> RSMAEEVSTLMKATVLMRQPGRVQEIVGALRKGGGDRLQVISDFDMTLSRFAYNG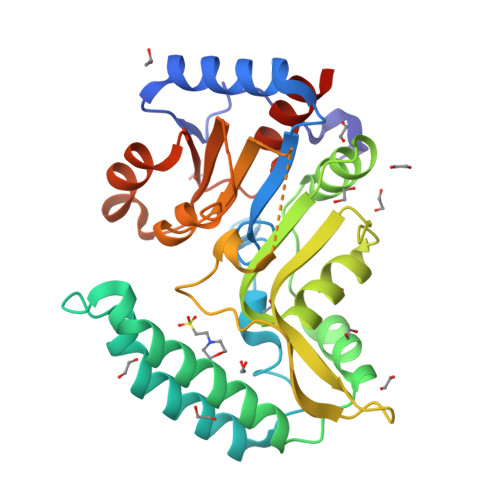KRCPSSYNILDNSKIISEECRKELTALLHHYYPIEIDPHRTVKEKLPHMVEWWTKAHNLLCQQKIQKFQIAQVVRESNAMLREGYKTFFNTLYHNNIPLFIFSAGIGDILEEIIRQMKVFHPNIHIVSNYMDFNEDGFLQGFKGQLIHTYNKNSSACENSGYFQQLEGKTNVILLGDSIGDLTMADGVPGVQNILKIGFLNDKVEERRERYMDSYDIVLEKDETLDVVNGLLQHILCQGVQLEMQGP>MAKLETVTLGNIGKD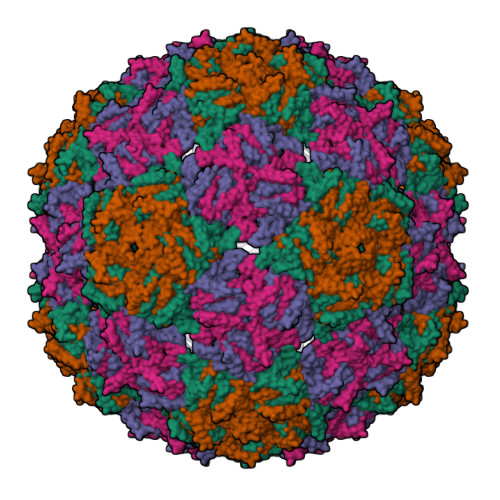GKQTLVLNPRGVNPTNGVASLSQAGAVPALEKRVTVSVSQPSRNRKNYKVQVKIQNPTACTANGSCDPSVTRQAYADVTFSFTQYSTDEERAFVRTELAALLASPLLIDAIDQLNPAY[4x]2-methyl-11-(1-methylethyl)-8-[(2S)-tetrahydro-2H-pyran-2-yl]-2,11,12,13-tetrahydro-4H-indazolo[5,4-a]pyrrolo[3,4-c]carbazol-4-one | C28 H28 N4 O2 | 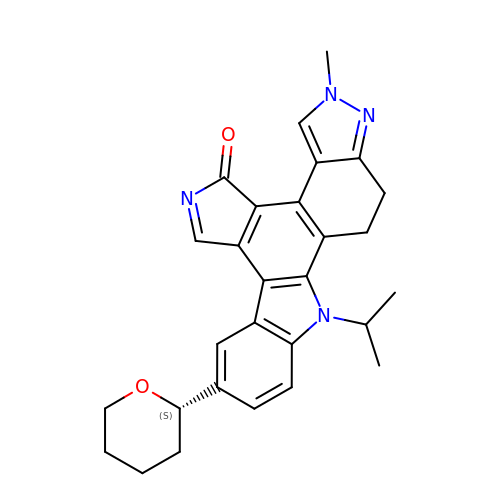JPKZOLAMWIKKME-QHCPKHFHSA-N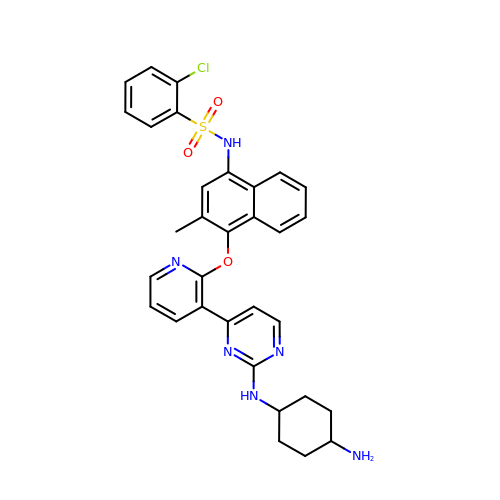N-{4-[(3-{2-[(trans-4-aminocyclohexyl)amino]pyrimidin-4-yl}pyridin-2-yl)oxy]-3-methylnaphthalen-1-yl}-2-chlorobenzenesulfonamide | C32 H31 Cl N6 O3 S | VMXTWHCDROGRNY-HZCBDIJESA-N>[6x]MATKGTKRSYEQMETDGERQNATEIRASVG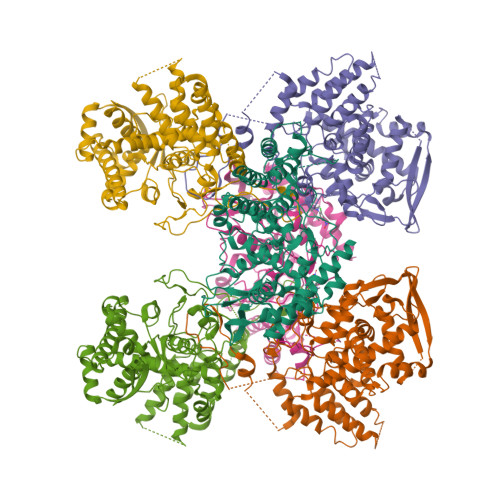KMIDGIGRFYIQMCTELKLSDYEGRLIQNSLTIERMVLSAFDERRNKYLEEHPSAGKDPKKTGGPIYRRVDGKWRRELILYDKEEIRRIWRQANNGDDATAGLTHMMIWHSNLNDATYQRTRALVRTGMDPRMCSLMQGSTLPRRSGAAGAAVKGVGTMVMELIRMIKRGINDRNFWRGENGRRTRIAYERMCNILKGKFQTAAQRTMVDQVRESRNPGNAEFEDLIFLARSALILRGSVAHKSCLPACVYGSAVASGYDFEREGYSLVGIDPFRLLQNSQVYSLIRPNENPAHKSQLVWMACHSAAFEDLRVSSFIRGTKVVPRGKLSTRGVQIASNENMETMESSTLELRSRYWAIRTRSGGNTNQQRASSGQISIQPTFSVQRNLPFDRPTIMAAFTGNTEGRTSDMRTEIIRLMESARPEDVSFQGRGVFELSDEKATSPIVPSFDMSNEGSYFFGDNAEEYDN>[6x]MSELFS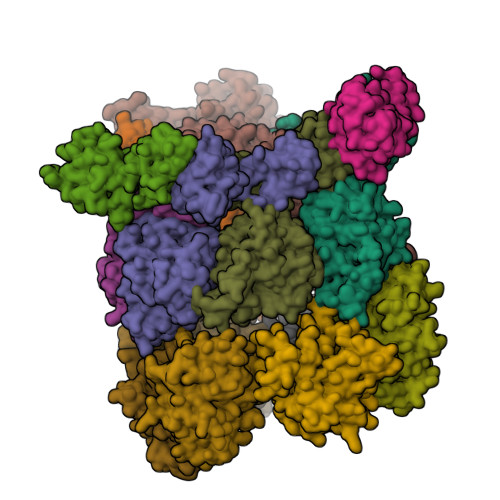ERIPPQSIEAEQAVLGAVFLDPAALVPASEILIPEDFYRAAHQKIFHAMLRVADRGEPVDLVTVTAELAASEQLEEIGGVSYLSELADAVPTAANVEYYARIVEEKSVLRRLIRTATSIAQDGYTREDEIDVLLDEADRKIMEVSQRKHSGAFKNIKDILVQTYDNIEMLHNRDGEITGIPTGFTELDRMTSGFQRSDLIIVAARPSVGKTAFALNIAQNVATKTNENVAIFSLEMSAQQLVMRMLCAEGNINAQNLRTGKLTPEDWGKLTMAMGSLSNAGIYIDDTPSIRVSDIRAKCRRLKQESGLGMIVIDYLQLIQGSGRSKENRQQEVSEISRSLKALARELEVPVIALSQLSRSVEQRQDKRPMMSDIRESGSIEQDADIVAFLYRDDYYNKDSENKNIIEIIIAKQRNGPVGTVQLAFIKEYNKFVNLERRFDEAQIPPGA;>KLLPAFQNAERLLLAHMMRSRDVALVVQERIGGRFNIEEHRALAAYIYAFYEEGHEADPGALISRIPGELQPLASELSLLLIADDVSEQELEDYIRHVLNRPKWLMLKVKEQEKTEAERRKDFLTAARIAKEMIEMKKMLSSS[3x];>[6x]MEPIGRSLQGVTGRPDFQKRLEQMKEKVMKDQDVQAFLKENEEVIDQKMIEKSLNKLYEYIEQSKNCSYCSEDENCNNLLEGYHPKLVVNGRSIDIEYYECPVKRKLDQQKKQQSLMKSMYIQQDLLGATFQQVDISDPSRLAMFQHVTDFLKSYNETGKGKGLYLYGKFGVGKTFMLAAIANELAEKEYSSMIVYVPEFVRELKNSLQDQTLEEKLNMVKTTPVLMLDDIGAESMTSWVRDEVIGTVLQHRMSQQLPTFFSSNFSPDELKHHFTYSQRGEKEEVKAARLMERILYLAAPIRLDGENRRHPHHHHHH> MANPNYFTYFRYGNNLGLTPIENYADQFRIEAGGKLNSVKPVPTATDAKDGLSSLKWEVELKHNPNNTKATINESTGQITITGLKQGQCGMVMVTATAGEGKTAVSVKQPVFFHFSMISDSNVQLEYTPFVFQVNPARGGESIAPSLGAGIDKSTFRLDYRRDFFYYNIAGPDSHISGALAQKVDNF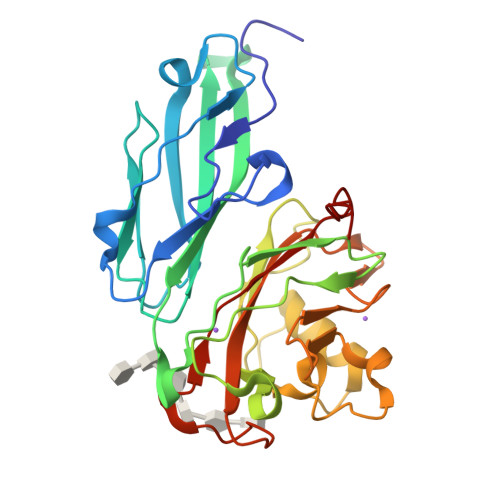LSEMWNSYDATAGTSRKPMSYFENTTNLSKALGYIDQTDFKVHINPNLWRNKDGYANGAMIGQITYDVTGKDPQAATSGARVSPIFIWFDTKFLEHHHHHH>[6x]MPTLPKAEAKELSAFVQSCVEYKTNVCFTDVAAYESNQKGVLSSGLAVLVGTHKQLRDPAVQRLPFYNPAVAEAIERVKEGGTYGVLVEGLANAAGSKFVRVVVGEVPTKASRNNCPARPDVVTALVTAALDEVKEPNTTVDVFVLSNAVLPIAAAVARCGKHNFSAKDGAAAAAYNSGKVSRLQVVFPEPPAIPPKDLEAVATSTQLCQRLVDAPPNLLTTATFTEIAQGYAKALGFDVDVICGDDLCERGYGGIYSVGKAAFEAPRLVTLLYTPKGTPVKKVSLVGKGIVYDCGGLALKPADYMKLMKHDMGGAAAVFCGFLTAVRLQQPVQLSCTLCLAENAIGPKSYRNDDIIVMKSGKTVEVINTDAEGRIVLGDGVFHATNELSFTPDVVIDMATLTGAQGIATGRHHAGLYVNEEGAEAAMLRAGRESGETCFPVLYCPEYHEPEFKSNHADMTNLMERRDNAGVSCAGYFITTHLSPKFTGAHIHVDLAYPVFNSNGATGFGPALLTEYFRKL

Leucine aminopeptidase (LAP) is found in all kingdoms of life and catalyzes the metal-dependent hydrolysis of the N-terminal amino acid residue of peptide or amino acyl substrates. We report here the X-ray structures of three kinetoplastid acidic LAPs (LAP-As from Trypanosoma brucei, Trypanosoma cruzi, and Leishmania major) which were solved in the metal-free and unliganded forms, as well as in a number of ligand complexes, providing insight into ligand binding, metal ion requirements, and oligomeric state. LAPs of the M17 family of aminopeptidases are bilobal proteins with a highly conserved C-terminal domain harboring the aminopeptidase activity. They form homohexamers of approximately 330 kDa with the active sites facing a central cavity separated from the bulk solvent but accessible through solvent channels.

TbLAP-A crystals in space group P212121 with six chains in the asymmetric unit grew under citrate-containing conditions and comprise apo TbLAP-A with no metal ions in the active site. All attempts to cryoprotect the crystals prior to vitrification resulted in substantial loss of diffraction quality, and only the apo TbLAP-A crystals were successfully cryoprotected. The structures of LAP-As in their apo and holo forms and in complex with inhibitors are practically identical. The exception is the metal-free apo TbLAP-A form, whose active-site loop (aa 293 to 305) is disordered and in which no electron density for bound metal ions could be detected, most likely because of the high concentration of citrate in the crystallization buffer.>[4x]HHHHHHFNLPPGNYKKPKLLYCSNGGHFLRILPDGTVDGT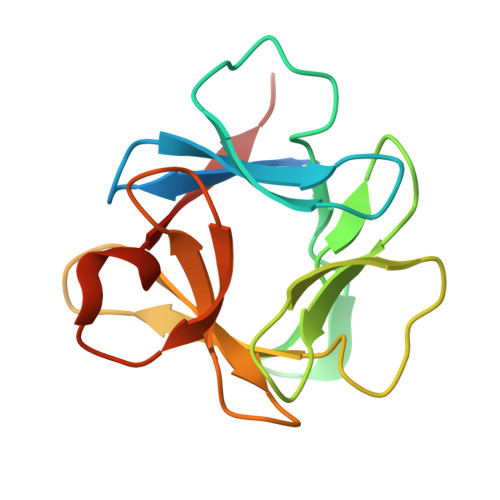RDRSDQHIQFQLSAESVGEVYIKSTETGQYLAIDTDGLVYGSQTPNEECLFLERLEENHYNTYISKKHGWYLGIKKNGSVKGTHYGQKAILFLPLPVSSD> LDFQALEETTEYDGGYTRDSVLIREFWEIVHSFTDEQKRLFLQFTTGT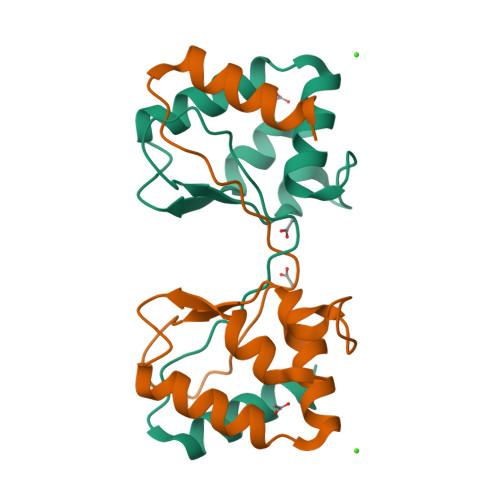DRAPVGGLGKLKMIIAKNGPDTERLPTSHTCFNVLLLPEYSSKEKLKERLLKAITYA> HMELALNVTESFDAWENTVTEQAIEDVWQLFETSIKP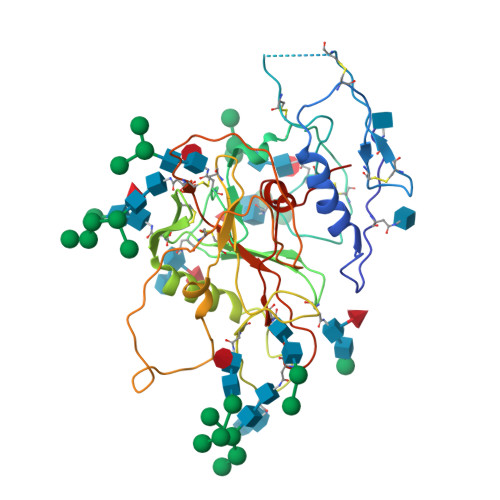CVKLSPLCIGAGHCNTSIIQESCDKHYWDTIRFRYCAPPGYALLRCNDTNYSGFMPKCSKVVVSSCTRMMETQTSTWFGFNGTRAENRTYIYWHGRDNRTIISLNKYYNLTMKCRGAGWCWFGGNWKDAIKEMKQTIVKHPRYTGTNNTDKINLTAPRGGDPEVTFMWTNCRGEFLYCKMNWFLNWVEDRDVTNQRPKERHRRNYVPCHIRQIINTWHKVGKNVYLPPREGDLTCNSTVTSLIANIDWTDGNQTNITMSAEVAELYRLELGDYKLVEIT> GACC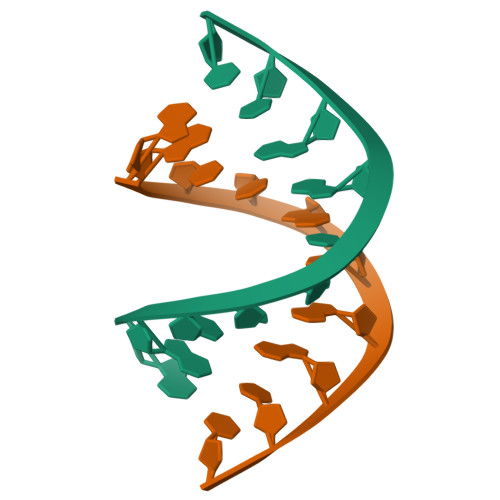GCGGTC>MILKERQDGVLVLTLNRPEKLNAITGELLDALYAALKEGEEDRE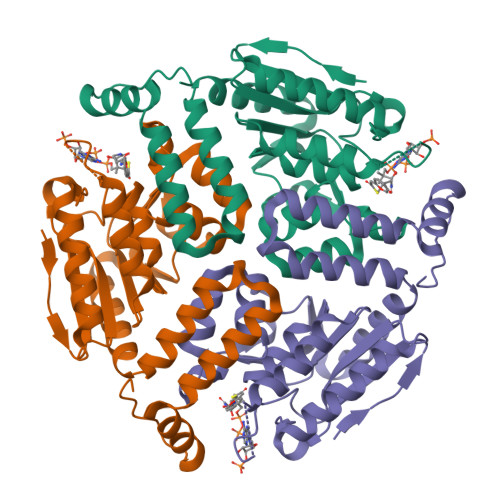VRALLLTGAGRAFSAGQDLTEFGDRKPDYEAHLRRYNRVVEALSGLEKPLVVAVNGVAAGAGMSLALWGDLRLAAVGASFTTAFVRIGLVPNSGLSFLLPRLVGLAKAQELLLLSPRLSAEEALALGLVHRVVPAEKLMEEALSLAKELAQGPTRAYALTKKLLLETYRLSLTEALALEAVLQGQAGQTQDHEEGVRAFREKRPPRFQGR[6x]>MIFSVDKVRADFPVLSREVNGLPLAYLDSAASAQKPSQVIDAEAEFYRHGYAAVHRGIHTLSAQATEKMENVRKRASLFINARSAEELVFVRGTTEGINLVANSWGNSNVRAGDNIIISQMEHHANIVPWQMLCARVGAELRVIPLNPDGTLQLETLPTLFDEKTRLLAITHVSNVLGTENPLAEMITLAHQHGAKVLVDGAQAVMHHPVDVQALDCDFYVFSGHKLYGPTGIGILYVKEALLQEMPPWEGGGSMIATVSLSEGTTWTKAPWRFEAGTPNTGGIIGLGAALEYVSALGLNNIAEYEQNLMHYALSQLESVPDLTLYGPQNRLGVIAFNLGKHHAYDVGSFLDNYGIAVRTGHHCAMPLMAYYNVPAMCRASLAMYNTHEEVDRLVTGLQRIHRLLG[2x];>MALLPDKEKLLRNFLRCANWEEKYLYIIELGQRLPELRDEDRSPQNSIQGAQSQVWIVMRQNAQGIIELQGDSDAAIVKGLIAVVFILYDQMTPQDIVNFDVRPWFCKMALTQHLTPSRSQGLEAMIRAIRAKAAALS[2x]

The cysteine desulfurase, SufS, provides sulfur in the SUF Fe-S cluster bioassembly pathway. SufS is a dimeric, pyridoxal 5'-phosphate-dependent enzyme that uses cysteine as a substrate to generate alanine and a covalent persulfide on an active site cysteine residue. SufS enzymes are activated by an accessory transpersulfurase protein, either SufE or SufU depending on the organism, which accepts the persulfide product and delivers it to downstream partners for Fe-S assembly. Due to the buried nature of the active site, these enzymes require a dedicated accessory protein called a transpersulfurase to act as a second substrate in the reaction.

Here, we report the first costructure for the SufS–SufE complex from E. coli. We obtained crystals of SufE C51A/E107C bound to SufS and solution of this structure indicated an EcSufS/EcSufE complex with 1:1 stoichiometry between the S and E subunits. The crystals diffracted anisotropically to 3.2 Å along the b-axis and c-axis, but to only 4.2 Å along the a-axis. The overall structure contains one EcSufE monomer per EcSufS active site and is asymmetric with one EcSufE positioned closer to the EcSufS active site, though neither pairing is in a persulfide transfer ready position. The overall asymmetry is best described as a rotation of EcSufE toward EcSufS resulting in a closure of approximately 7°. The more open interaction is based primarily on contacts between EcSufE and the α16 helix (residues 343–353) of EcSufS, while the closure creates additional interactions between the C51 and R119 loops on EcSufE and the R56 loop and α4 helix of the adjacent SufS monomer. H343, D346, and Y354 of EcSufS hydrogen bond to D74, backbone amides of A76 and I77, and E21 on EcSufE, respectively. The remainder of the α16 helix interface is made up of nonpolar interactions between EcSufE and Y345 and F350 on EcSufS. The EcSufE residues in these contacts are located in the C51 loop (residues 47–53) and the R119 loop and flanking regions (residues 112–128); however, the loop surrounding R119 (residues 116–120) lacks density in both EcSufE subunits. These two regions form layered interactions with the N terminus of the α4 helix (residues 60–67) and the adjacent R56 loop (residues 56–59) on EcSufS, with R56 appearing to block formation of a closer complex.Postsynaptic scaffold proteins such as Shank, PSD-95, Homer and SAPAP/GKAP family members establish the postsynaptic density of glutamatergic synapses through a dense network of molecular interactions. In the presence of Zn2+, the SAM-domain polymerizes into helical fibers, which may be stacked side-by-side through interhelical contacts. This enables the formation of large sheets where Shank proteins multimerize, allowing Shank proteins to serve as building blocks in deeper layers of the PSD.

Upon solving the structure of the WT, we observed high similarity between the Shank2-SAM domain, and the structure of M56E mutant Shank3-SAM domain. Though no Zn2+ was added to Shank2 crystals, we observed that about 30% of the Zn2+ sites were occupied. Apparently some Zn2+ binding had been maintained during purification. Due to the incomplete occupancy, the tetrahedral coordination of the Zn2+ ion made by His1803, His1835, a chloride ion and Glu1802 was somewhat distorted and incomplete. Nevertheless, the WT SAM domain crystallized in the same space group, showing the same crystal packing as reported for Shank3. Importantly, this packing arrangement allowed for the formation of helical polymers of SAM domains, and the side-by-side alignment of these helices, leading to larger sheets of polymerized SAM domains. As reported by [13], contacts via the intrahelical interface can be distinguished from the additional inter-polymer interface. Both interfaces are supported by the Zn2+ binding site which is localized at the contact site between these two interfaces. A closer inspection of the interactions of SAM domains within the crystals showed that the WT domain established several interactions with the neighboring molecules, which are responsible for the formation of helical fibers. In addition, we observed interactions to SAM domains in the neighboring helix.

> TKPVHLWTKPDVADWLESLNLGEHKEAFMDNEIDGSHLPNLQKEDLIDLGVTRVGHRMNIERALKQLLDR> MKKVRLKELESRLQQVDGFEKPKLLLEQYPTRPHIAACMLYTIHNTYDDIENKVVADLGCGCGVLSIGTAMLGAGLCVGFDIDEDALEIFNRNAEEFELTNIDMVQCDVCLLSNRMSKSFDTVIMNPPFGTKNNKGTDMAFLKTALEMARTAVYSLHKSSTREHVQKKAAEWKIKIDI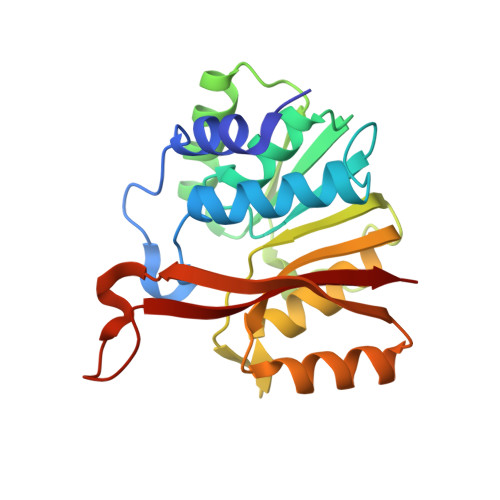IAELRYDLPASYKFHKKKSVDIEVDLIRFSF>TETTSFLITKFSPDQQNLIFQGDGYTTKEKLTLTKAVKNTVGRALYSSPIHIWDRETGNVANFVTSFTFVINAPNSYNVADGFTFFIAPVDTKPQTGGGYLGVFNSAEYDKTTETVAVEFDTFYNAAWDPSNRDRHIGIDVNSIKSVNTKSWKLQNGEEANVVIAFNAATNVLTVSLTYP[2x];>VTSYTLSDVVSLKDVVPEW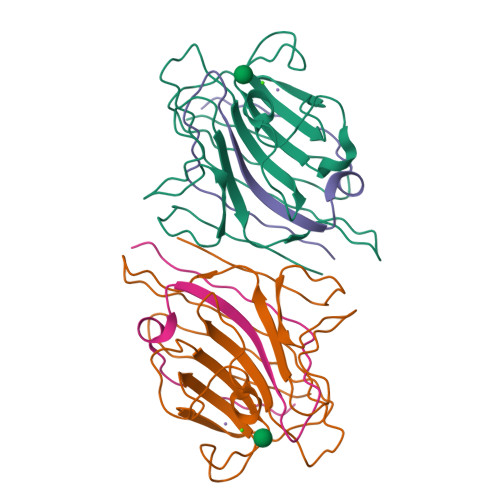VRIGFSATTGAEYAAHEVLSWSFHSELSGT[2x]~{N}4-ethyl-~{N}2,~{N}4-dimethyl-~{N}2-(1-methylpiperidin-4-yl)quinazoline-2,4-diamine 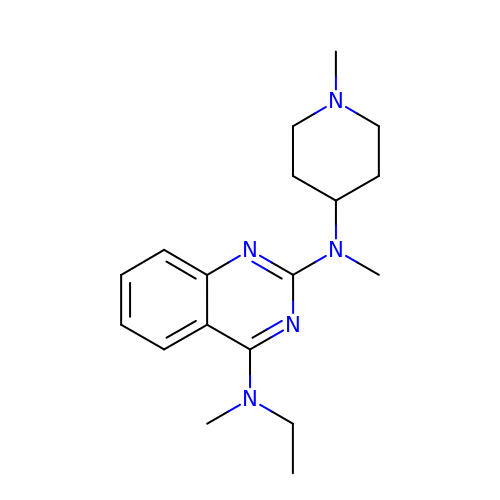| C18 H27 N5 | SNYUVAMIFMFCIL-UHFFFAOYSA-N> EVKQENRLLNESESSSQGLLGYYFSDLNFQAPMVVTSSTTGDLSIPSSELENIPSENQYFQSAIWSGFIKVKKSDEYTFATSADNHVTMWVDDQEVINKASNSNKIRLEKGRLYQIKIQYQRENPTEKGLDFKLYWTDSQNKKEVISSDNLQLPELKQKSSNSRK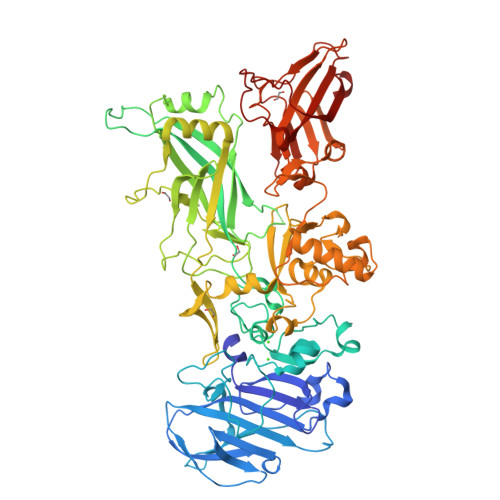KRSTSAGPTVPDRDNDGIPDSLEVEGYTVDVKNKRTFLSPWISNIHEKKGLTKYKSSPEKWSTASDPYSDFEKVTGRIDKNVSPEARHPLVAAYPIVHVDMENIILSKNEDQSTQNTDSQTRTISKNTSTSRTHTSEVHGNAEVHASFFDIGGSVSAGFSNSNSSTVAIDHSLSLAGERTWAETMGLNTADTARLNANIRYVNTGTAPIYNVLPTTSLVLGKNQTLATIKAKENQLSQILAPNNYYPSKNLAPIALNAQDDFSSTPITMNYNQFLELEKTKQLRLDTDQVYGNIATYNFENGRVRVDTGSNWSEVLPQIQETTARIIFNGKDLNLVERRIAAVNPSDPLETTKPDMTLKEALKIAFGFNEPNGNLQYQGKDITEFDFNFDQQTSQNIKNQLAELNATNIYTVLDKIKLNAKMNILIRDKRFHYDRNNIAVGADESVVKEAHREVINSSTEGLLLNIDKDIRKILSGYIVEIEDTEGLKEVINDRYDMLNISSLRQDGKTFIDFKKYNDKLPLYISNPNYKVNVYAVTKENTIINPSENGDTSTNGIKKILIFSKKGYEIG>MVANTTYKAPIERPEDFLKDKEKAKEWERKEAERIEQKLERSEKEALESYKKDSVEISKYSQTRNYFYDYQIEANSREKEYKELRNAISKNKIDKPMYVYYFESPEKFAFNKVIRTENQNEISLEKFNEFKETIQNKLFKQDGFKDISLYEPGKGDEKPTPLLMHLKLPRNTGMLPYTNTNNVSTLIEQGYSIKIDKIVRIVIDGKHYIKAEASVVSSLDFKDDVSKGDSWGKANYNDWSNKLTPNELADVNDYMRGGYTAINNYLISNGPVNNPNPELDSKITNIENALKREPIPTNLTVYRRSGPQEFGLTLTSPEYDFNKLENIDAFKSKWEGQALSYPNFIFTSIGSVNMSAFAKRKIVLRITIPKGSPGAYLSAIPGYAGQYQVLLNHGSKFKINKIDSYKDGTIT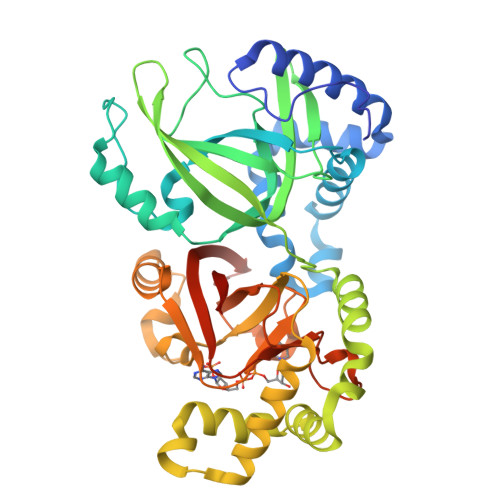KLIVDATLIPLEHHHHHH[4x]> GAGCAGACCCG;> ACGGCACTCA;> CGCGT;> TCTGAGTGCGGT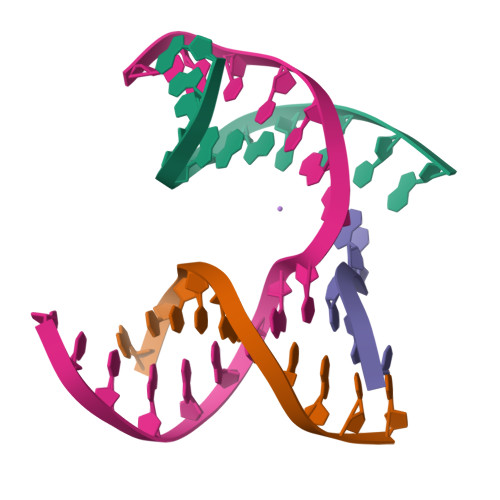CTGC>GPGSEFELRRQMAERAALEELVKLQGERVRGLKQQKASAELIEEEVAKLLKLKAQLGPDESKQKFVLKTPKGTRDYSPRQMAVREKVFDVIIRCFKRHGAEVIDTPVFELKETLMGKYGEDSKLIYDLKDQGGELLSLRYDLTVPFARYLAMNKLTNIKRYHIAKVYRRDNPAMTRGRYREFYQCDFDIAGNFDPMIPDAECLKIMCEILSSLQIGDFLVKVNDRRILDGMFAICGVSDSKFRTICSSVDKLDKVSWEE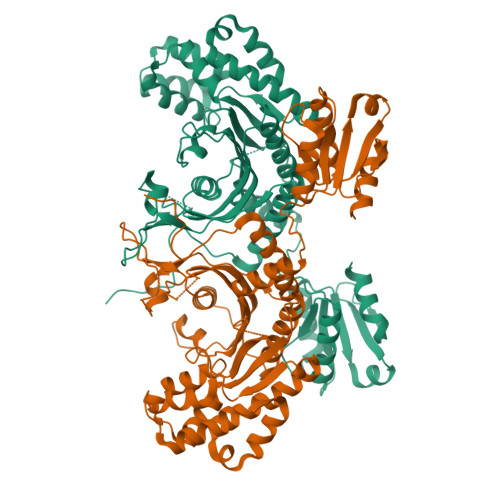VKNEMVGEKGLAPEVADRIGDYVQQHGGVSLVEQLLQDPKLSQNKQALEGLGDLKLLFEYLTLFGIDDKISFDLSLARGLDYYTGVIYEAVLLQTPAQAGEEPLGVGSVAAGGRYDGLVGMFDPKGRKVPCVGLSIGVERIFSIVEQRLEALEEKIRTTETQVLVASAQKKLLEERLKLVSELWDAGIKAELLYKKNPKLLNQLQYCEEAGIPLVAIIGEQELKDGVIKLRSVTSREEVDVRREDLVEEIKRRTGQPL[2x]>[4x]GSHMKPASFMTSICDERGQELIYAGMPITEVFKEEMGIGGVLGLLWFQKRLPKYSCQFI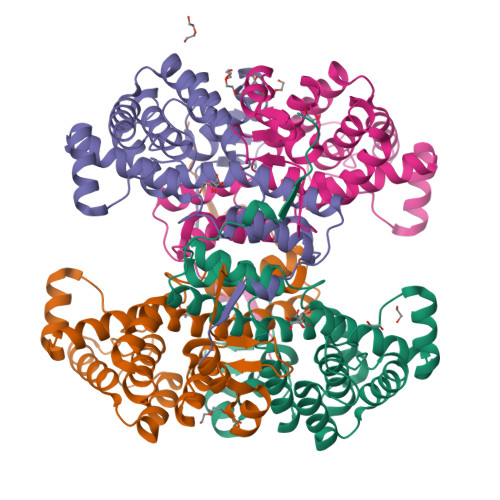EMCLMVTADHGPAVSGAHNTIICARAGKDLVSSLTSGLLTIGDRFGGALDAAAKMFSKAFDSGIIPMEFVNKMKKEGKLIMGIGHRVKSINNPDMRVQILKDYVRQHFPATPLLDYALEVEKITTSKKPNLILNVDGLIGVAFVDMLRNCGSFTREEADEYIDIGALNGIFVLGRSMGFIGHYLDQKRLKQGLYRHPWDDISYVLPEHMSM> MKPERKRVSKLMAYILRHSPEEFGLRPDV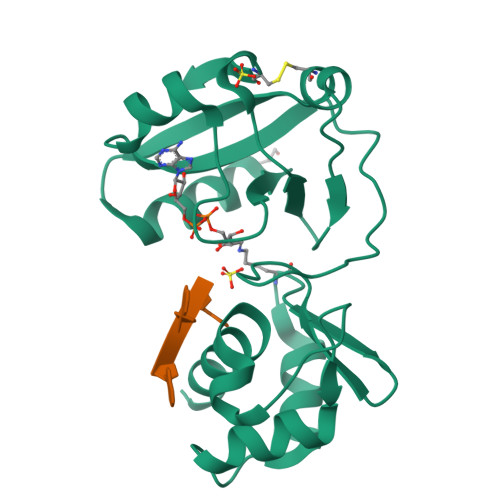EGFVSLNELVNALKTVYPEVTEEFVREIVENDPXGRYEIRGDRIRARYGHSFPVSLDHEEDTESRFLYHGTPRRNLPSILKEGLKPMKRQYVHVSTDKIEALETGRRHGREVVLLVIDAECLRKRGFKIYKAGKNVRIVERVPPDCITLAV> MHHHHHHMIEWIIRRSVANRFLVLMGALFLSIWGTWTIINTPVDALPDLSDVQVIIKTSYPGQAPQIVENQVTYPLTTTMLSVPGAKTVRGFSQFGDSYVYVIFEDGTDPYWARSRVLEYLNQVQGKLPAGVSAELGPDATGVGWIYEYALVDRSGKHDLADLRSLQDWFLKYELKTIPDVAEVASVGGVVKEYQVVIDPQRLAQYGISLAEVKSALDASNQEAGGSSIELAEAEYMVRASGYLQTLDDFNHIVLKASENGVPVYLRDVAKVQIGPEMRRGIAELNGEGEVAGGVVILRSGKNAREVIAAVKDKLETLKSSLPEGVEIVTTYDRSQLIDRAIDNLSGKLLEEFIVVAVVCALFLWHVRSALVAIISLPLGLCIAFIVMHFQGLNANIMSLGGIAIAVGAMVAAAIVMIENAHKRLEEWQHQHPDATLDNKTRWQVITDASVEVGPALFISLLIITLSFIPIFTLEGQEGRLFGPLAFTKTYAMAGAALLAIVVIPILMGYWIRGKIPPESSNPLNRFLIRVYHPLLLKVLHWPKTTLLVAALSVLTVLWPLNKVGGEFLPQINEGDLLYMPSTLPGISAAEAASMLQKTDKLIMSVPEVARVFGKTGKAETATDSAPLEMVETTIQLKPQEQWRPGMTMDKIIEELDNTVRLPGLANLWVPPIRNRIDMLSTGIKSPIGIKVSGTVLADIDAMAEQIEEVARTVPGVASALAERLEGGRYINVEINREKAARYGMTVADVQLFVTSAVGGAMVGETVEGIARYPINLRYPQSWRDSPQALRQLPILTPMKQQITLADVADIKVSTGPSMLKTENARPTSWIYIDARDRDMVSVVHDLQKAIAEKVQLKPGTSVAFSGQFELLERANHKLKLMVPMTLMIIFVLLYLAFRRVGEALLIISSVPFALVGGIWLLWWMGFHLSVATGTGFIALAGVAAEFGVVMLMYLRHAIEAVPSLNNPQTFSEQKLDEALYHGAVLRVRPKAMTVAVIIAGLLPILWGTGAGSEVMSRIAAPMIGGMITAPLLSLFIIPAAYKLMWLHRHRV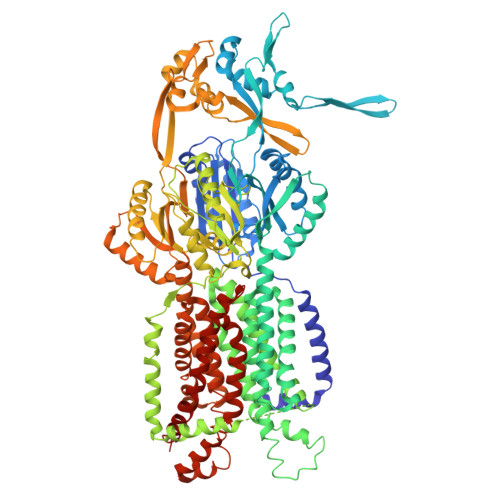RK> SIPPVKAGAKQLPMPSVSGAQIKLLGADYEQLVNSKGKIAPVISDTPVNVS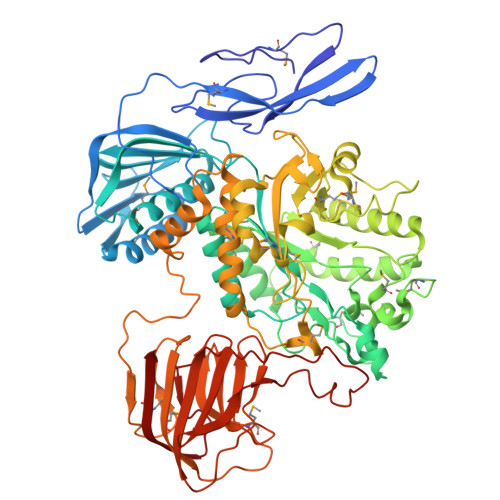FKVTKDGKEAVSKDYEIMLQAPQAAQGNPKPRIIPEILQWKGGQGEYKLGNTVTIACPDKELGKLFAADMEDVLGKKVKLVAPGAKADISLSLLKGGNLGREGYRLQIARDGVRLGAAAPTGLFWGTRTLLQMLRQTPGSVPCGTAVDFPRYQLRGFMLDVARTPYPLSYLKDVIRTMAWYKMNDLHLVINNNYIFHEHYVDNGHDPFKESYAAFRLESKMKGKDGTPLTARDLFYTKKEFADLVSYARKYGVNIVPEFDTPGHALSFTRLRPDLIYKGPMNHEKRRCEMLDAANPETIDLVSKVFDEYMLKDPKLGRPVFADCGVVHVGADEFYGDKEDYRHFANAVLTHALKRGYTPRIWGSLSAKPGKTPVVSKGVQMNLWSTGWMKAWEAVNQGYDVINTNDGALYIVPFAGYYRMDRNHKGLYNNWIPNRIGNETLPSGHPQLLGGTFAVWNDETDIMHTGYAPYDIWGIISGSMDVLSQKLWGTAKAPDTFEQHRELVSSIGNAPRTNPLHKWKDSQPLTVKPSSLPQKLDKPALGPNYRLTMELELTAAPEGKEQVLLAAPEGELLAVMKDGTVGFRRDDSLEFSFGAKLPVGKKVKVEIVGEPEKTSLLLDGEPAGTAVLKNFSDKSKDFSDKFKHRPKVHRSTFILPLKELGSSFQGKVFHMNVQPL> MDYKDDDDKGGGWSHPQFEKGGGMSDSASNTEDSIQIEIFPSRILSPETAQKLISELYQVDGIIRVMVQGPRLPERVSAGPGTGEKVEHPLRKPIQIGDQVIELKISVGRIRLEIENAETKEKVRSVCDKMLPFSFEFREGHFLRRKPT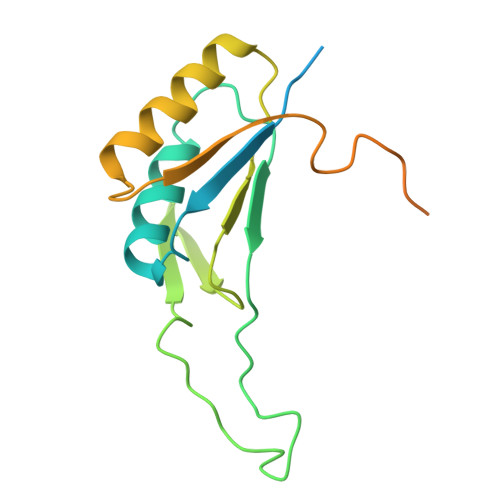VTDYAKLGPETDPRLLGMVDPKAKVNQLVFIEKREKEDDTDKDE>[5x]GQDMVSPPPPIADEPLTVNTGIYLIESYSLDDKAETFKVNAFLSLSWKDRRLAFDPVRSGVRVKTYEPEAIWIPEIRFVNVENARDADVVDISVSPDGTVQYLERFSARVLSPLDFRRYPFDSQTLHIYLIVRSVD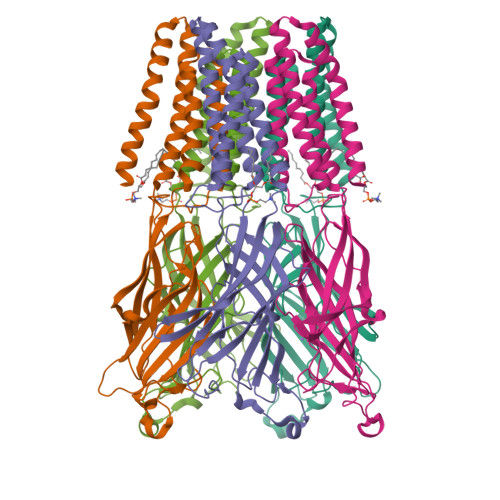TRNIVLAVDLEKVGKNDDVFLTGWDIESFTAVVKPANFALEDRLESKLDYQLRISRQYFSYIPNWILPMLFILFISWTAFWSTSYEANVTLVVSTLIAHIAFNILVCTNLPKTPYMTYTGAIIFMIYLFYFVAVIEVTVQHYLKVESQPARAASITRASRIAFPVVFLLANIILAFLFFGF1-methylpyrrolidine-2,5-dione | C5 H7 N O2 | 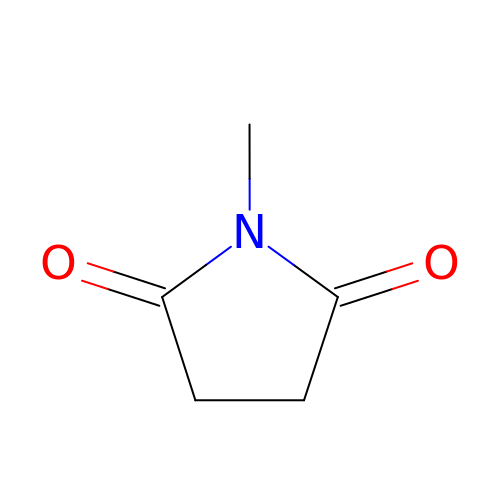KYEACNNYFNZCST-UHFFFAOYSA-N>MAKDIGINSDPNSSSVDKLMKSSGVSNPTYTLVWKVWILAVTLYFAIRIPLTLVFPSLFSPLLPLDILASLALIADIPLDLAFESRRTSGRKPTLLAPSRLPDLLAALPLDLLVFALHLPSPLSLLSLVRLLKLISVQRSATRILSYRINPALLRLLSLVGFILLAAHGIACGWMSLQPPSENPAGTRYLSAFYWTITTLTTIGYGDITPSTPTQTVYTIVIELLGAAMYGLVIGNIASLVSKLDAAKLLHRERVERVTAFLSYKRISPELQRRIIEYFDYLWETRRGYEEREVLKELPHPLRLAVAMEIHGDVIEKVPLFKGAGEEFIRDIILHLEPVIYGPGEYIIRAGEMGSDVYFINRGSVEVLSADEKTRYAILSEGQFFGEMALILRAPRTATVRARAFCDLYRLDKETFDRILSRYPEIAAQIQELAVRRKELESSGLVPRGSVKHHHH[4x]

Here, we used SthK, a cyclic nucleotide-modulated channel from Spirochaeta thermophila, to define a ligand-gating trajectory that includes multiple on-pathway intermediates. cAMP is a poor partial agonist for SthK and depolarization increases SthK activity. CNG channels are tetrameric channels where each subunit consists of a voltage sensing domain (VSD, S1–S4), a pore domain (S5-S6), and a cytosolic cyclic nucleotide binding domain (CNBD) that is linked to the pore domain via a C-linker comprised of four α helices. Meanwhile, membrane depolarization increases cAMP-induced channel activity, suggesting that voltage modulates the agonist status of cAMP in SthK, similar to its action on other CNG channels, although the mechanism is not known. Cryo-EM structures of VSD mutants with increased activity yielded cAMP-bound closed states (identical to apo and cAMP-bound WT SthK), as well as four additional states: one gating intermediate and 3 open states with different degrees of opening.

Tyr26 is located on the S1 helix, and its hydroxyl group is coordinated by the guanidine group of Arg111, a conserved arginine in the S4 helix and presumably important for voltage sensing in SthK. Removal of the hydroxyl group, as in SthK Y26F, abolishes this interaction, which can conceivably facilitate S4 movement in the membrane. SthK Y26F adopts two conformations in the presence of cAMP. The majority of particles (1112621 particles, ~91%) was in a closed conformation, identical to the closed state of WT SthK (RMSD = 0.4 Å) as expected from our functional data (Po at 0 mV is ~0.25). Importantly, the Y26F mutation does not lead to any local or other changes in the channel as gleaned from the identical structures of WT SthK and SthK Y26F in the closed state. In all three open conformations of SthK R120A, the lower two helical turns of the S4 helix of the VSD are displaced outwards by a small kink at Val118, allowing S5 to move, which creates space for the expansion of S6. This lateral displacement is not observed in the closed states, which show identical S4 helices in SthK WT, Y26F, and R120A. In the closed state, the bundle crossing is stabilized by an inter-subunit salt-bridge between Arg136 on S5 and Asp226 on S627. In both cases, SthK Y26F and SthK R120A, the mutation did not lead to different protein conformations at rest but altered the relative stabilities between closed and open states.> GSHMQ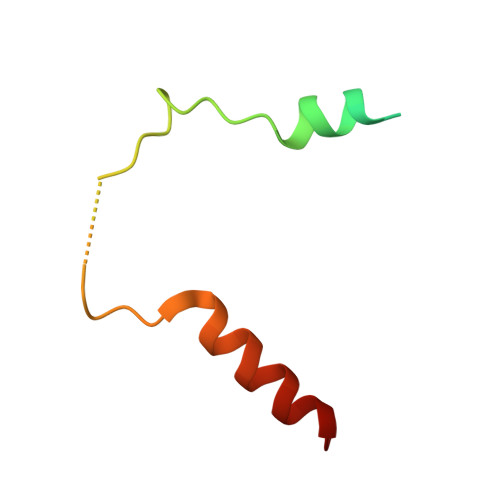KGQVGIFSFQNNYADSATTFRILAHLDEQRYPLPNGAAEKNLPSLFEGFKATVSIIQQR>MVMKNHLHTIMEDWKLSGTALMKKGEDIPFIASLGFANRAERIPNEHHTRFGIASGCKLFTAIAICQLVEAGKLSFDTPLSDWLDAPFPNVTIHHLLTHTSGVPDYFDEEITDDFEDLWKDVPMYHLRRLKDFLPLFQHAPMKFPPGHRFHYNNAGFILLGLVVESVSGVTFQEYVEANVFQRAGMHESGYFAFDTLPAKTALGYIDLEDGSWKTNLYSLPVIGGSDGGAYVTAEDMMKLWLALMRHELLNETYTQKLLTPHVHCEDDD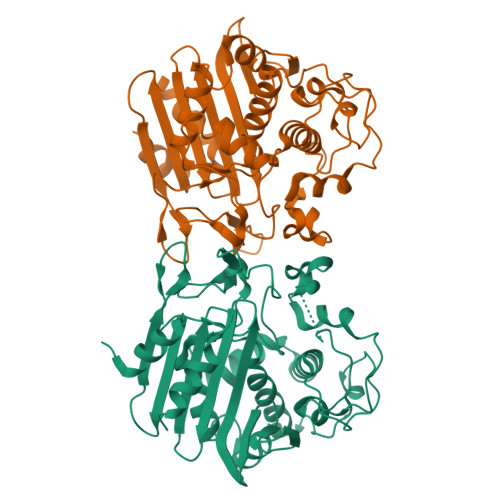YYGYGVWIKQQDGAISKYHVMGYDPGVCFHSAFYPTSNGIVVVCANQSSGAYDVMAAIEALFSEAAENLYFQSHHHHHHWSHPQFEK[2x]> MSLGAKPFGEKKFIEIKGRRMAY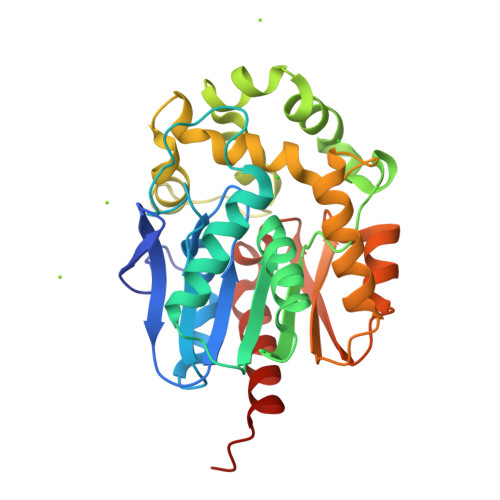IDEGTGDPILFQHGNPTSSYLWRNIMPHCAGLGRLIACDLIGMGDSDKLDPSGPERYAYAEHRDYLDALWEALDLGDRVVLVVHDWGSALGFDWARRHRERVQGIAYMEAIAMPIEWADFPEQDRDLFQAFRSQAGEELVLQDNVFVEQVLPGLILRPLSEAEMAAYREPFLAAGEARRPTLSWPRQIPIAGTPADVVAIARDYAGWLSESPIPKLFINAEPGALTTGRMRDFCRTWPNQTEITVAGAHFIQEDSPDEIGAAIAAFVRRLRPAHHHHHH To gain structural insights into a putative complex formed by FtsH and YidC, we performed single-particle cryogenic electron microscopy on detergent-solubilized membrane samples, from which FtsH and YidC were purified using Ni–NTA affinity and size-exclusion chromatography. Although SDS–PAGE analysis indicated high purity of these proteins, cryo-EM data sets unexpectedly yielded high-resolution structures of ArnA and AcrB at 4.0 and 2.9 Å resolution, respectively. ArnA is a bifunctional enzyme involved in lipid A modification and polymyxin resistance, while AcrB is a multidrug efflux transporter of the AcrAB–TolC system. ArnA and AcrB, known Ni–NTA purification contaminants, were also consistently detected by mass spectrometry in Strep-Tactin affinity-purified samples, validating their presence independently of affinity-tag selection.

ArnA is a bifunctional enzyme that catalyzes the biosynthesis of 4-amino-4-deoxy-l-arabinose (l-Ara4N), a nucleotide-activated sugar that is incorporated into lipid A to reduce its net negative charge and thereby enhance resistance to cationic antimicrobial peptides such as polymyxins. In terms of domain organization, ArnA is a bifunctional cytoplasmic enzyme composed of two catalytic domains: an N-terminal transformylase domain, which catalyzes the formylation of UDP-4-amino-4-deoxy-l-arabinose (UDP-Ara4N), and a C-terminal dehydrogenase domain, which catalyzes the nicotinamide adenine dinucleotide, oxidized form (NAD+)-dependent decarboxylation of UDP-glucuronic acid. These domains are connected by a flexible linker and act sequentially in the Ara4N biosynthesis pathway. For ArnA, 123 593 particles were processed through heterogeneous and non-uniform refinement, initially using C1 symmetry and later D3 symmetry. The final atomic model comprised 12 chains and 3726 residues, reflecting the hexameric organization of ArnA. Additional variations were observed in other surface-exposed loops, suggesting local flexibility or alternative domain orientations that may be influenced by differences in sample conditions or oligomeric assembly. A previous study has shown that ArnA can adopt multiple oligomeric forms, including hexamers and tetramers, and undergoes conformational changes upon substrate binding. Although ArnA was not detectable by Coomassie-stained SDS–PAGE, single-particle cryo-EM analysis yielded a 4.0 Å resolution reconstruction, which currently constitutes the highest resolution cryo-EM structure of this protein available in both the EMDB and PDB.

>MKTVVFAYHDMGCLGIEALLAAGYEISAIFTHTDNPGEKAFYGSVARLAAERGIPVYAPDNVNHPLWVERIAQLSPDVIFSFYYRHLIYDEILQLAPAGAFNLHGSLLPKYRGRAPLNWVLVNGETETGVTLHRMVKRADAGAIVAQLRIAIAPDDIAITLHHKLCHAARQLLEQTLPAIKHGNILEIAQRENEATCFGRRTPDDSFLEWHKPASVLHNMVRAVADPWPGAFSYVGNQKFTVWSSRVHPHASKAQPGSVISVAPLLIACGDGALEIVTGQAGDGITMQGSQLAQTLGLVQ[6x];>[6x]MRVLILGVNGFIGNHLTERLLREDHYEVYGLDIGSDAISRFLNHPHFHFVEGDISIHSEWIEYHVKKCDVVLPLVAIATPIEYTRNPLRVFELDFEENLRIIRYCVKYRKRIIFPSTSEVYGMCSDKYFDEDHSNLIVGPVNKPRWIYSVSKQLLDRVIWAYGEKEGLQFTLFRPFNWMGPRLDNLNAARIGSSRAITQLILNLVEGSPIKLIDGGKQKRCFTDIRDGIEALYRIIENAGNRCDGEIINIGNPENEASIEELGEMLLASFEKHPLRHHFPPFAGFRVVESSSYYGKGYQDVEHRKPSIRNAHRCLDWEPKIDMQETIDETLDFFLRTVDLTD> MTSTAVEITVKNAADIAIIGGSGLYQMQALTNKRSVKIETPYGEPSDDIVLGELNGVTVAFLTRHGQGHRLTPSEVPYRANIYALKTLGVRYIVSVSAVGSLQETLKP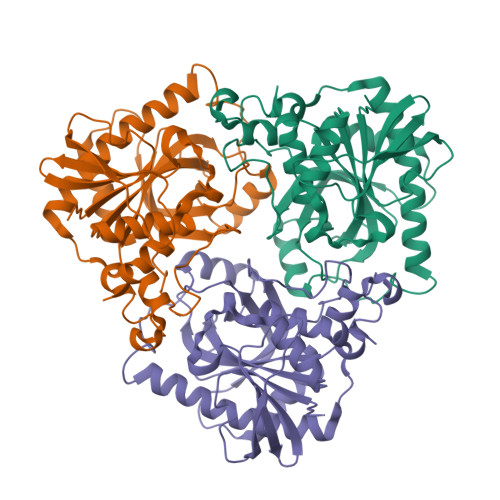LDMVIPDQMIDMTKQRVSTFFGDGAVAHVSMADPLCPEVADILIRAYDNADIADGQCHAKATYVCIEGPQFSTRAESHWYRQMQADIIGMTNMPEAKLAREASIAYATLALVTDFDCWHPNEQAVSADYAIQNLMKNADNAQQVIKQAVALIASEQPKSIAHTALTQALVTPVEAMSAETKTRLAALLP> GNETIVQCESMTKGG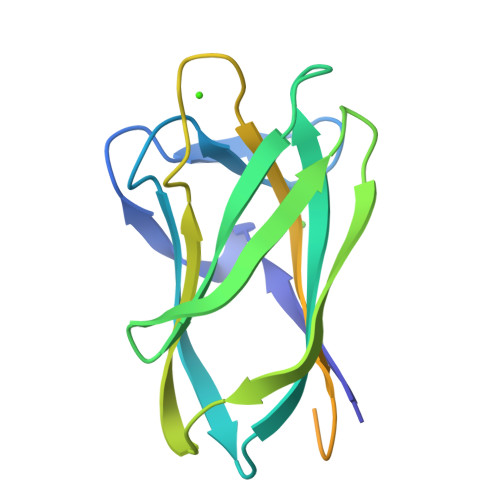QYTGNINNPFGGVALYGNNDKVSYTQYFASGTHDFTLRGCSNNDNMARVDLKIGGETKGTFYYGGSSPAEYTIKNVNHGTGNQTIELVVTADNGQWDANIDYLKIGGAGVGGNESSGGNQGGNEGNQGGNAGNEGGNQAGNTGNQGGNEGNAGGQHHHHHH>MAHHHHHHEVLFQGPGAKKRKMYEDILSHVNILKDMDPYERCKVADCLKSKSYNDGEIIIKEGEEGDTFFILIDGNAVASKDNKVIKTYTKGDYFGELALL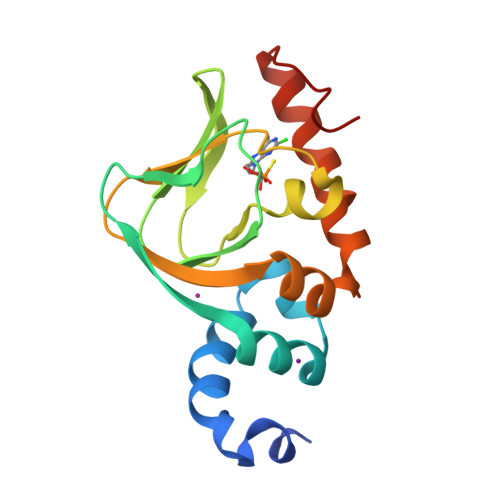KNKPRAATIKAQNFCQVVYLDRKSFKRLLGPIEDILHRNVENYKKVLNELGLDTTCIDEN[2x]2-{[3-(decyloxy)benzoyl]amino}-5-nitrobenzoic 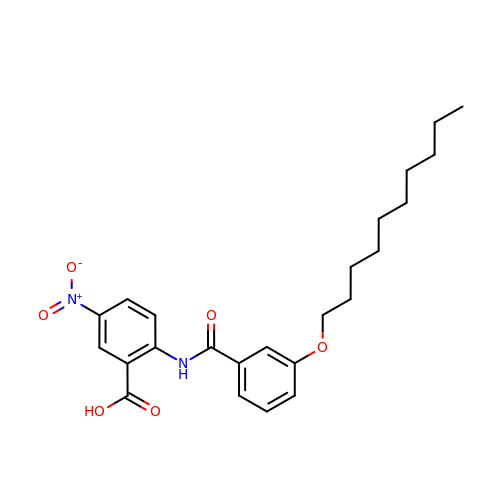acid | C24 H30 N2 O6 | PZXIQAYPKSOMHD-UHFFFAOYSA-N> MTKRDHNKVYNVTLVNEERG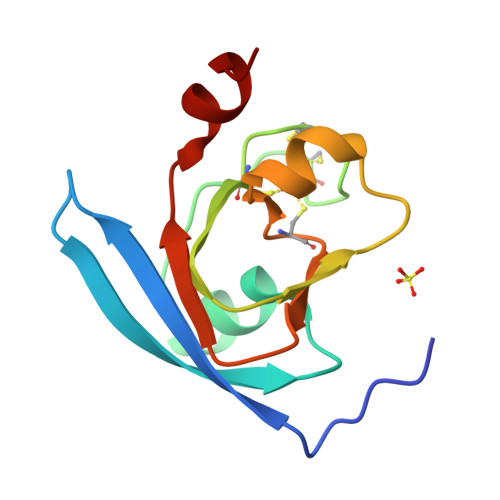LNKTIRVHADEYILDAAEAQGIPLPYSCRAGACVNCAGRIIKGTVDQSDHSFLKPKELDAGFVLLCAAYPTSDCVISTHEEDNLLNLA>MILNNQEWLLAIFKKKGLTPTGKLEFATIDGIDSALAQALNEAFDSQVVSFNDRINQSFREFLKRTPRDRITLGTFSDVKEWLSSFEADRAGRKDTASAGPVNKLAMPLVNLSRSPAFSIYEGELCRDNYDEGHVTNENDEIEALVSTIPFSLEYSLWIASDEKESLGMVTTALAFWLRMYASLGQASFTHIANVGGYEIPVTCYI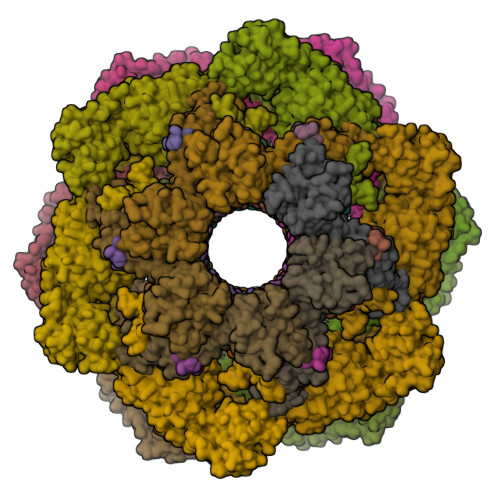EGQKSIAFQDLTTGTADNRLFAVGLNLTVVAELPILAYMQQTTGTITVKAKILEE[6x];>MGHNNTKGNRKFIKGRYTANAAKGERLVSSEFLLTFAGHEDISVLVRTSQIPEMTREDVEDYGPNGVKFNQHGPIRNSGEIQVQCVETIEGDILQFIKDRIAAKDYVDITMAATPESKSSGVNAVTKAATTIEMLDCKIYSDAIDFSTEDVTAAVRPSLRIVYNWIEWD[12x];>[12x]MSQYSIQQSLGNASGVAVSPINADATLSTGVALNSSLWAGIGVFARGKPFTVLAVTESNYEDVLGEPLKPSSGSQFEPIRHVYEAIQQTSGYVVRAVPDDAKFPIIMFDESGEPAYSALPYGSEIELDSGEAFAIYVDDGDPCISPTRELTIETATADSAGNERFLLKLTQTTSLGVVTTLETHTVSLAEEAKDDMGRLCYLPTALEARSKYLRAVVNEELISTAKVTNKKSLAFTGGTNGDQSKISTAAYLRAVKVLNNAPYMYTAVLGLGCYDNAAITALGKICADRLIDGFFDVKPTLTYAEALPAVEDTGLLGTDYVSCSVYHYPFSCKDKWTQSRVVFGLSGVAYAAKARGVKKNSDVGGWHYSPAGEERAVIARASIQPLYPEDTPDEEAMVKGRLNKVSVGTSGQMIIDDALTCCTQDNYLHFQHVPSLMNAISRFFVQLARQMKHSPDGITAAGLTKGMTKLLDRFVASGALVAPRDPDADGTEPYVLKVTQAEFDKWEVVWACCPTGVARRIQGVPLLIK>[4x]HHMSAIKPDMK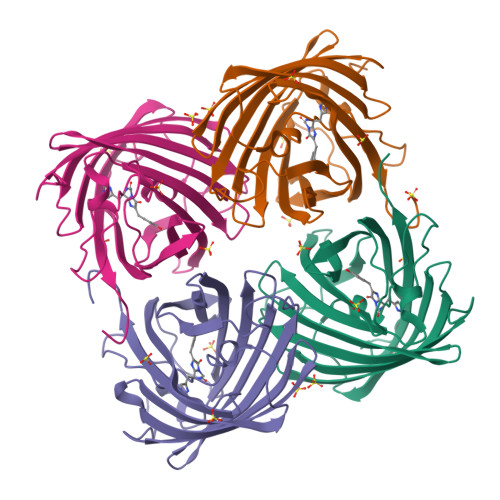INLRMEGNVNGHHFVIDGDGTGKPFEGKQSMDLEVKEGGPLPFAFDILTTAFHYGNRVFAEYPDHIQDYFKQSFPKGYSWERSLTFEDGGICIARNDITMEGDTFYNKVRFHGVNFPANGPVMQKKTLKWEPSTEKMYVRDGVLTGDITMALLLEGNAHYRCDSRTTYKAKEKGVKLPGYHLVDHCIEILSHDKDYNKVKLYEHAVAHSGLPDNARR>[2x]MPNASQVYRSTRSSSPKTISFEEAIIQGLATDGGLFIPPTIPQVDQATLFNDWSKLSFQDLAFAIMRLYIAQEEIPDADLKDLIKRSYSTFRSDEVTPLVQNVTGDKENLHILELFHGPTYAFKDVALQFVGNLFEYFLQRTNANLPEGEKKQITVVGATSGDTGSAAIYGLRGKKDVSVFILYPTGRISPIQEEQMTTVPDENVQTLSVTGTFDNCQDIVKAIFGDKEFNSKHNVGAVNSINWARILAQMTYYFYSFFQATNGKDSKKVKFVVPSGNFGDILAGYFAKKMGLPIEKLAIATNENDILDRFLKSGLYERSDKVAA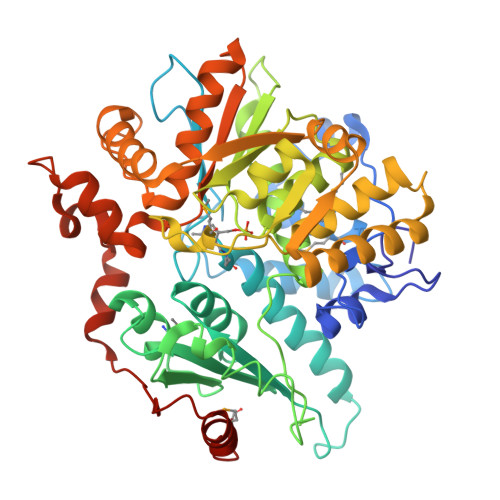TLSPAMDILISSNFERLLWYLAREYLANGDDLKAGEIVNNWFQELKTNGKFQVDKSIIEGASKDFTSERVSNEETSETIKKIYESSVNPKHYILDPHTAVGVCATERLIAKDNDKSIQYISLSTAHPAKFADAVNNALSGFSNYSFEKDVLPEELKKLSTLKKKLKFIERADVELVKNAIEEELAKMKL> TSASGPEHEFVS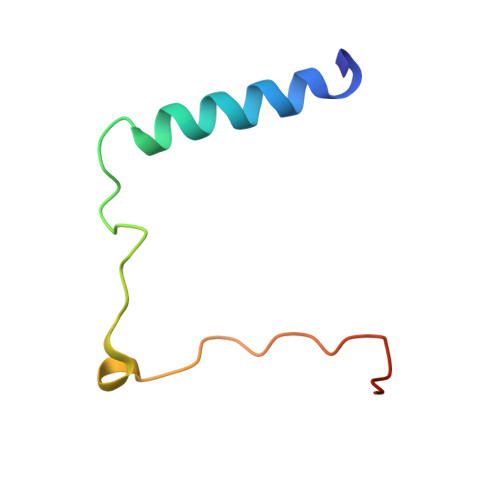KFLTLATLTEPKLPKSYTKPLKDVTNLGVPLPTLKYKYKQNR> MPVAGSELPRRPLPPAAQERDAEPRP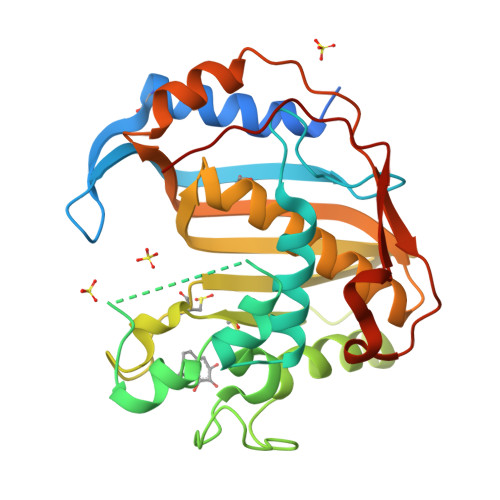PHGELQYLGQIQHILRCGVRKDDRTGTGTLSVFGMQARYSLRDEFPLLTTKRVFWKGVLEELLWFIKGSTNAKELSSKGVKIWDANGSRDFLDSLGFSTREEGDLGPVYGFQWRHFGAEYRDMESDYSGQGVDQLQRVIDTIKTNPDDRRIIMCAWNPRDLPLMALPPCHALCQFYVVNSELSCQLYQRSGDMGLGVPFNIASYALLTYMIAHITGLKPGDFIHTLGDAHIYLNHIEPLKIQLQREPRPFPKLRILRKVEKIDDFKAEDFQIEGYNPHPTIKMEMAV Bacterial HSS is mostly found in α-proteobacteria and in some β- and γ-proteobacteria, including pathogenic strains such as Legionella pneumophila, Brucella spp. and various P. aeruginosa strains, including PA7 and PA14. It catalyzes the conversion of two molecules of putrescine (PUT; 1,4-diaminobutane) into one molecule of sym-homospermidine [HSP; bis(4-aminobutyl)amine] as the main reaction along with several side reactions (Ober et al., 1996; Böttcher et al., 1994). Bacterial HSS is NAD+-dependent, active at neutral to basic pH with an optimum at pH ∼8.8, and shows increased activity in the presence of 50 mM potassium ion. BvHSS forms a dimer, with each subunit containing a boot-shaped substrate-binding pocket between an NAD(P)-binding Rossmann-like domain and an HSS-like domain. The cofactor NAD+ is bound as a prosthetic group in the binding pocket with its nicotinamide ring being part of the active site.

More evidence for cation–π interaction as a requirement for efficient catalysis might be inferred from the inactive variant W229A. The ‘inner’ amino group of both PUT molecules is similarly placed near the carboxyl group of Glu210. The ‘outer’ amino group in the W229A variant, however, is shifted towards or attracted by the carboxyl group of Glu237 (distance 3.3 Å) compared with the wild-type protein (distance 4.4 Å). In context of the oxidation of PUT C4 by NAD+ as part of the proposed reaction mechanism, the distance between PUT C4 and NAD+ C4N is 4.4 Å in the variant and 2.2 Å in the wild-type structure. An explanation for the inactivity of the W229A variant could therefore be the missing cation–π interaction, which prevents appropriate stabilization of the ‘outer’ amino group of PUT at the ‘center amino site’ near the nicotinamide ring. This could ultimately impede hydride transfer between PUT C4 and the nicotinamide ring as a prerequisite for imine formation. However, the lack of a bulky, confining side chain at position 229 broadens the active site and might thereby allow increased flexibility of the PUT molecule. This could also contribute to the inappropriate positioning of the PUT molecule in this variant, preventing further conversion of the substrate.

>[2x]GPMGTDWPVYHRIDGPIVMIGFGSIGRGTLPLIERHFAFDRSKLVVIDPSDEARKLAEARGVRFIQQAVTRDNYRELLVPLLTAGPGQGFCVNLSVDTSSLDIMELARENGALYIDTVVEPWLGFYFDPDLKPEARSNYALRETVLAARRNKPGGTTAVSCCGANPGMVSWFVKQALVNLAADLGVTGEEPTTREEWARLAMDLGVKGIHIAERDTQRASFPKPFDVFVNTASVEGFVSEGLQPAELGWGTFERWMPDNARGHDSGCGAGIYLLQPGANTRVRSWTPTAMAQYGFLVTHNESISIADFLTVRDAAGQAVYRPTCHYAYHPCNDAVLSLHEMFGSGKRQSDWRILDETEIVDGIDELGVLLYGHGKNAYWYGSQLSIEETRRIAPDQNATGLQVSSAVLAGMVWALENPNAGIVEADDLDFRRCLEVQTPYLGPVVGVYTDWTPLAGRPGLFPEDIDTSDPWQFRNVLVRD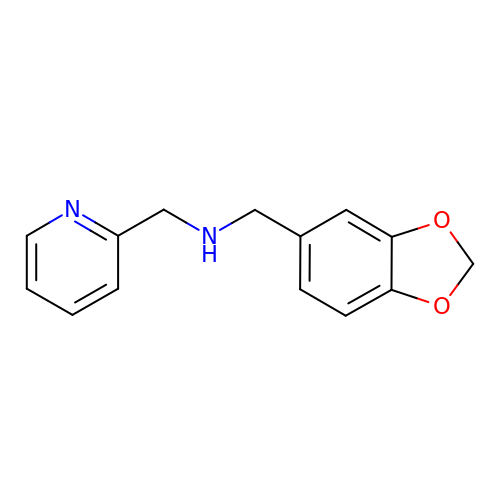1-(1,3-benzodioxol-5-yl)-~{N}-(pyridin-2-ylmethyl)methanamine | C14 H14 N2 O2 | KZQVJMBMNZMAGV-UHFFFAOYSA-N>ASATNDPRFDDLWGLNNEGQTGGTADADIDAPEAWSISTGSRDVVVGVIDTGVDYSHPDLAANAWVNSGEIAGDGIDNDGNGYIDDVHGINAITDVGDPMDDEGHGTHVSGTIGASGNNGVGVVGVNHDVSIVGCKFLAADGTGSTSGAIKCIDYMVGLKNAGVNLRVLNNSWGGGGFSQALADAITASEQADILFVAAAGNDAVDNDQNPHYPSNYENDNVLSIASTDSRDNMSSFSQWGLTSVDMGAPGSGILSTVPGNSYATYSGTSMATPHVAG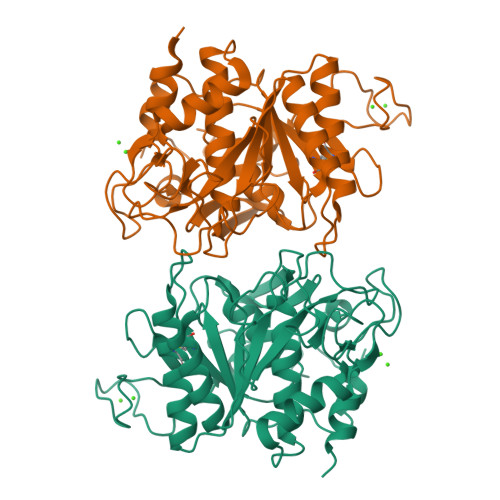AAALVLSVNPDLTTLELKELLMSSGDANAALNGKTVAGTRLNVNQALIDADPTPGF[2x]>GMSAPEDWNSQVIQEFRANGGRVGGNFEGAPMVLVHHVGRKTGKAAVTPMMYLPSDDDPGTIYVFASKAGAASNPAWYYNLTTAGTAQVEVGTETYAVGVTEVTGEDRDRIYSEQARRYPGFADYEKKTAGIRTIPVLALTRT[4x]

Herein, we describe the isolation and characterization of nine F420H2-dependent reductases (FDRs) from Mycobacterium smegmatis that utilize an F420H2 cofactor to catalyse the reduction of aflatoxins, leading to their spontaneous breakdown. Structural and phylogenetic analysis suggests that these nine enzymes fall into two hitherto unclassified enzyme families that are distantly related to the well characterized FMN-dependent pyridoxamine 5′-phosphate oxidase (PNPOx) family. The mechanism of aflatoxin breakdown appears to involve an initial, enzyme-catalysed reduction of the double bond of the α,β-unsaturated ester moiety, followed by spontaneous hydrolysis. Phylogenetic analysis of 146 PNPOx-like sequences, including 28 present in M. smegmatis, shows that the four proteins belong to two distinct families (< 12% amino acid identity), hereafter denoted FDR-A and -B (F420H2 dependent reductase -A and -B), which are both clearly differentiated from the functionally defined PNPOx family.

The three most active enzymes were from the FDR-A family (MSMEG_5998, 2850 and 3356). To gain further insight into the function of these newly identified enzymes, crystal structures of members of the FDR-A (MSMEG_3356) and FDR-B families (MSMEG_3380) were solved to 2.0 and 1.2 Å resolution respectively. MSMEG_3356 and MSMEG_3380 both adopt the PNPOx-like split barrel fold, comprising a central split barrel surrounded by four helices. MSMEG_3380 exists as a homodimer, while MSMEG_3356 is monomeric. Thus, it appears that MSMEG_3356 is the first characterized structure of a member of the FDR-A family. Despite their low similarity, the structures of both the FDRs described here are characterized by large hydrophobic pockets formed by several aromatic residues and a positively charged groove that is principally formed by several lysine and arginine side-chains. In terms of shape and electrostatic character, these pockets/channels are highly complementary to the F420H2 cofactor, which possesses an aromatic deazaflavin group and a long, negatively charged, side-chain consisting of a phospho-lactate and a variable number of glutamates. Consistent with the level of electrostatic and hydrophobic interactions implied by the docking results, titration curves of activity versus cofactor concentration show that both MSMEG_3356 and MSMEG_3380 bind F420H2 tightly, with apparent KM values in the nanomolar range (260 nM and 130 nM, respectively). In MSMEG_3356, the deazaflavin/substrate pocket is formed by W7, N25, F26, M31, P48, M49, M50, F64, A68, W76, F121 and Y124, and the positively charged groove is formed by the side-chains of N8, H36, R39, K40, T41, K43, T47 and K67. Also, the MSMEG_3380 cavity is significantly larger than that of MSMEG_3356 (649 Å3 versus 411 Å3).>MAPALNANPTTKRDELSAPSASHKLGMSSMASRAAGGGLKLTGLPDLSDSAGTLSDIFGTPQMREIWSDQNRVACYLEIEAALAIVQADLGIIPKNAAHEIVEHCRVQEIDWALYKQKTELIGYPVLGIVQQLVANCKDGLGEYCHWGATTQDITDTATVMQIRQSLTLVKQRLDSIVSSLEHLAEQHRNVPMAARSNLKQAVPITFGFKMARFLATFRRHQQRLVELEKRVYTLEFGGAAGNLSSLGDQGIATHDALAKMLDLAPAEIAWHTEHDRFAEVGTFLGLLTGTLAKLATDIKLMSQTEVGEVGEPFISNRGSSSTMPQKNNPISCVYIHACAANVRQGAAALLDAMQSDHERGTGPWEIIWVQLPLMMNWTSAALNNADFVLRGLQVFPDAMQHNLDLSKGLIVSEAVMMGLGNTLGRQYAHDAVYECCRTAFVQDRPLLDVLLE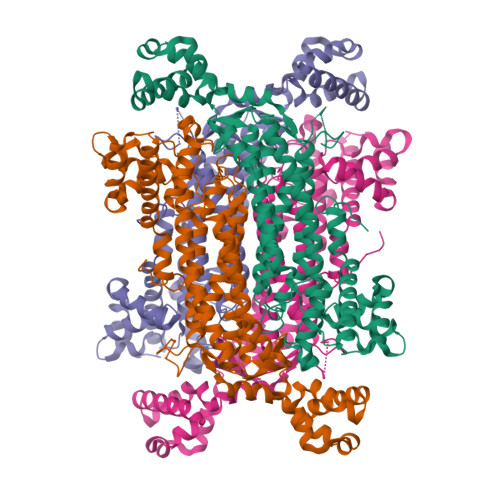NHEIASKLDRTELEKLCDPANYLGQCSQWIDRVLSPPSSA[4x]1-{4-[5-(3,4,5-trimethoxyphenyl)pyridin-3-yl]phenyl}piperazine | C24 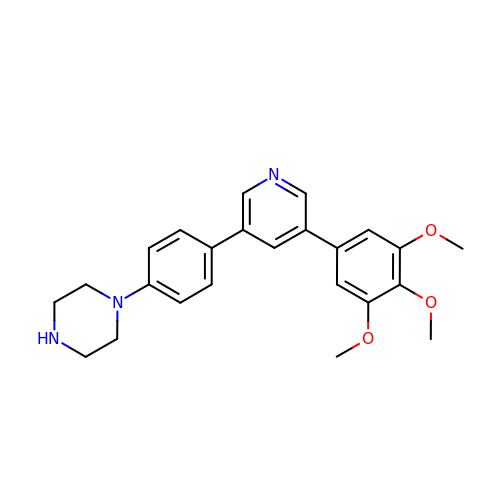H27 N3 O3 | WFZZPLAPENBNIY-UHFFFAOYSA-N> GHMSDSTESTNRFASNVRQAEAPNEKTLRIKVSALKRTIKDLEFAKREVERELQRLDTLCQSDPDRVPQQTKVVDEAQMMVPHSVNRI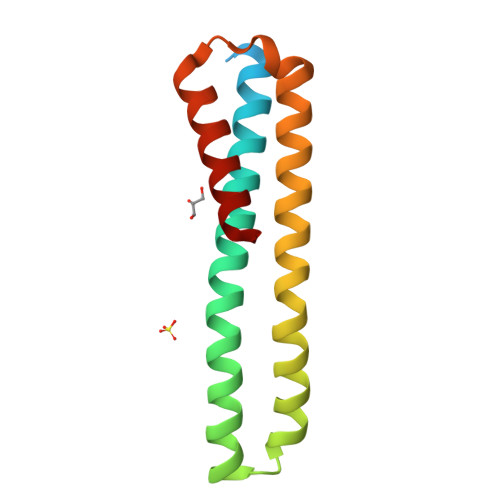MASVKDLSDYLEKEGSTVSNEELLDLARATMADGQAAVS> GSHMNTAEEDMEDDTSWRSEATFQ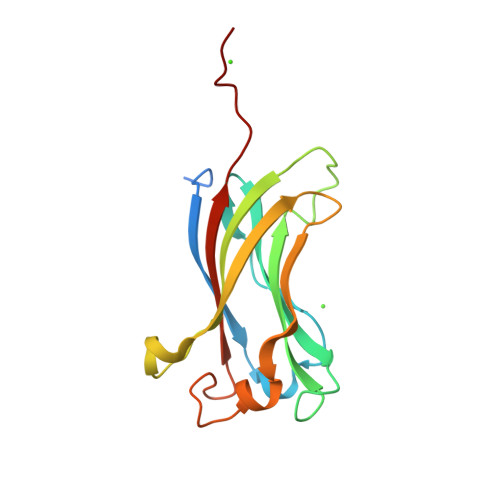FTVERFSRLSESVLSPPCFVRNLPWKIMVMPRFYPDRPHQKSVGFFLQCNAESDSTSWSCHAQAVLKIINYRDDEKSFSRRISHLFFHKENDWGFSNFMAWSEVTDPEKGFIDDDKVTFEVFVQADAPHGVAWD> APSFDCGKPQVEPKKCPGRVVGGCVAHPHSWPWQVSLRTRFGMHFCGGTLISPEWVLTAAHCLEKSPRPSSYKVILGAHQEVNLEPHVQEIEVSRLFLEPTRKDIALLKLSSPAVITDKVIPACLPSPNYVVADRTECFITGWGETQGTFGAGLLKEAQLPVIENKVCNRYEFLNGRVQSTELCAGHLAGGTDSCQGDSGGPLVCFEKDKYILQGVT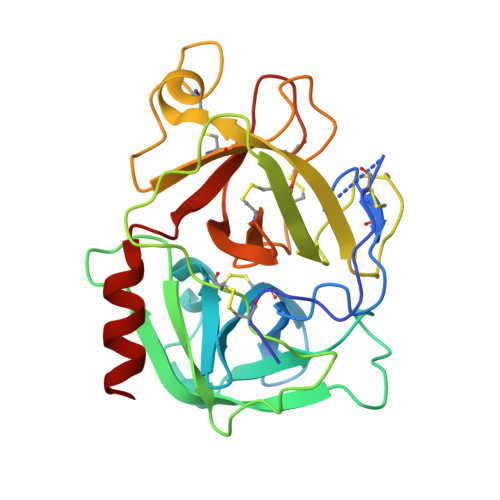SWGLGCARPNKPGVYVRVSRFVTWIEGVMRNN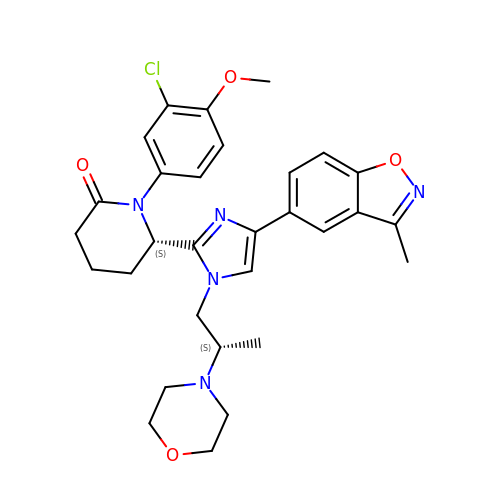(6~{S})-1-(3-chloranyl-4-methoxy-phenyl)-6-[4-(3-methyl-1,2-benzoxazol-5-yl)-1-[(2~{S})-2-morpholin-4-ylpropyl]imidazol-2-yl]piperidin-2-one | C30 H34 Cl N5 O4 | MPSAWTZVAUPXBG-SIBVEZHUSA-N> LKHIISAYNFSRDELEDIFALTDKYSKNLNDTRKILSGKTISIAFFEPSTRTYLSFQKAIINLGGDVIGFSGEESTSVAKGENLADTIRMLNNYSDGIVMRHKYD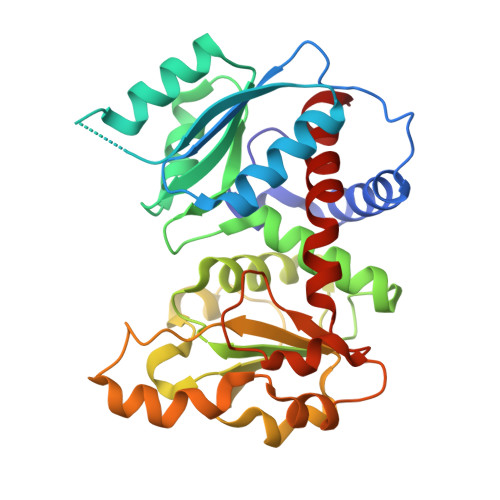GASRFASEISDIPVINAGDGKHEHPTQAVIDIYTINKHFNTIDGLVFALLGDLKYARTVNSLLRILTRFRPKLVYLISPQLLRARKEILDELNYPVKEVENPFEVINEVDVLYVTRIQKERFVDEMEYEKIKGSYIVSLDLANKMKKDSIILHPLPRVNEIDRKVDKTTKAKYFEQASYGVPVRMSILTKIYGE>AQDMVSPPPPIADEPLTVNTGIYLIECYSLDDKAETFKVNAFLSLSWKDRRLAFDP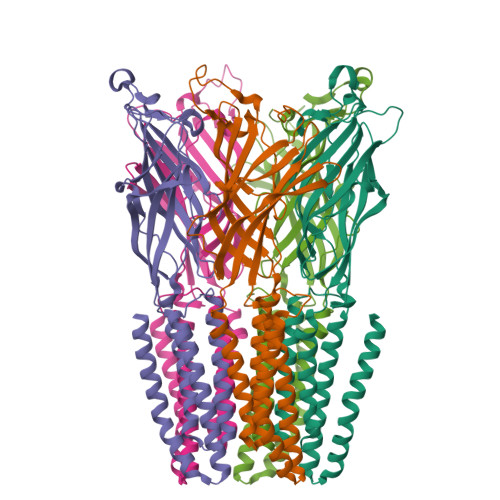VRSGVRVKTYEPEAIWIPEIRFVNVENARDADVVDISVSPDGTVQYLERFSARVLSPLDFRRYPFDSQTLHIYLIVRSVDTRNIVLAVDLEKVGKNDDVFLTGWDIESFTAVVKPANFALEDRLESKLDYQLRISRQYFSYIPNIILPMLFILFISWTAFWSTSYEANVTLVVSTLIAHIFFNILVETNLPKTPYMTYTGAIIFMIYLFYFVAVIEVTVQHYLKVESQPARAASITRASRIAFPVVFLLANIILAFLFFGF[5x]>MTSPVIGTPWKKLNAPVSEEALEGVDKYWRVANYLSIGQIYLRSNPLMK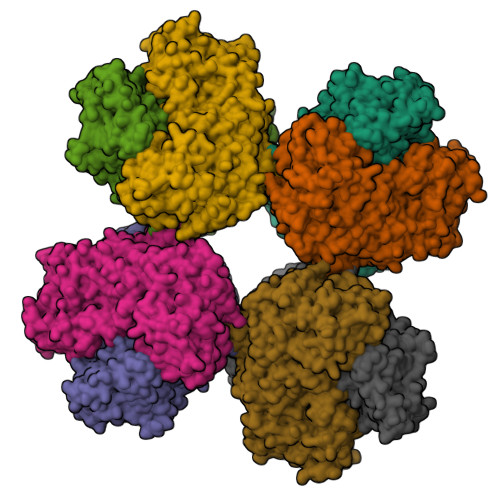EPFTREDVKHRLVGHWGTTPGLNFLIGHINRFIADHGQNTVIIMGPGHGGPAGTSQSYLDGTYTETFPKITKDEAGLQKFFRQFSYPGGIPSHFAPETPGSIHEGGELGYALSHAYGAIMDNPSLFVPAIVGDGEAETGPLATGWQSNKLVNPRTDGIVLPILHLNGYKIANPTILSRISDEELHEFFHGMGYEPYEFVAGFDDEDHMSIHRRFAELWETIWDEICDIKATAQTDNVHRPFYPMLIFRTPKGWTCPKYIDGKKTEGSWRSHQVPLASARDTEAHFEVLKNWLESYKPEELFDANGAVKDDVLAFMPKGELRIGANPNANGGVIRNDLKLPNLEDYEVKEVAEYGHGWGQLEATRTLGAYTRDIIKNNPRDFRIFGPDETASNRLQASYEVTNKQWDAGYISDEVDEHMHVSGQVVEQLSEHQMEGFLEAYLLTGRHGIWSSYESFVHVIDSMLNQHAKWLEATVREIPWRKPIASMNLLVSSHVWRQDHNGFSHQDPGVTSVLLNKCFHNDHVIGIYFATDANMLLAIAEKCYKSTNKINAIIAGKQPAATWLTLDEARAELEKGAAAWDWASTAKNNDEAEVVLAAAGDVPTQEIMAASDKLKELGVKFKVVNVADLLSLQSAKENDEALTDEEFADIFTADKPVLFAYHSYAHDVRGLIYDRPNHDNFNVHGYEEEGSTTTPYDMVRVNRIDRYELTAEALRMIDADKYADKIDELEKFRDEAFQFAVDNGYDHPDYTDWVYSGVNTDKKGAVTATAATAGDNEHHHHHH[8x]> HMEAQFFTDTGQHRDKNEDAGGIFYNQTNQQLLVLCDGMGGHKAGEVASKFVTDELKSRFEAENLIEQHQAENWLRNNIKDINFQLYHYAQENAEYKGMGTTCVCALVFEKSVVIANVGDSRAYVINSRQIEQITSDHSFVNHLVLTGQITPEEAFTHPQRNIITKVMGTDKRVSPDLFIKRLN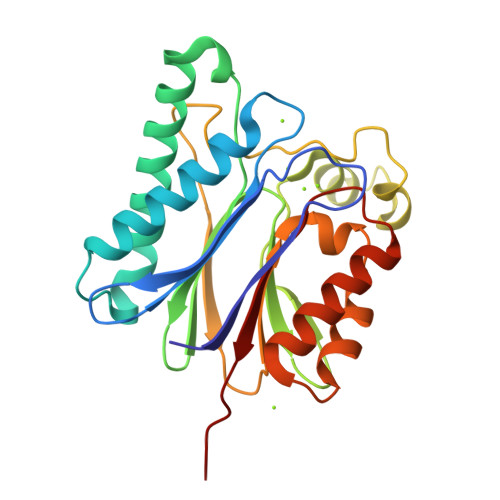FYDYLLLNSDGLTDYVKDNEIKRLLVKEGTIEDHGDQLMQLALDNHSKDNVTFILAAIEGDKV>[4x]AQTNIDVVPFNVAEGKEVLLVVHNESQNLYGYN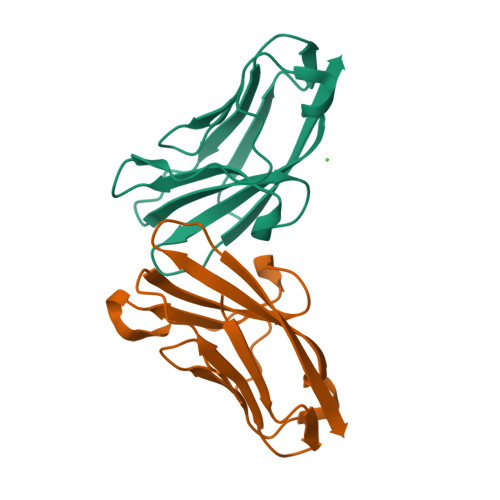WYKGERVHANYRIIGYVKNISQENAPGPAHNGRETIYPNGTLLIQNVTHNDAGIYTLHVIKENLVNEEVTRQFYVF>[2x]MTRTLPPGVSDERFDAALQRFRDVVGDKWVLSTADELEAFRDPYPVGAAEANLPSAVVSPESTEQVQDIVRIANEYGIPLSPVSTGKNNGYGGAAPRLSGSVIVKTGERMNRILEVNEKYGYALLEPGVTYFDLYEYLQSHDSGLMLDCPDLGWGSVVGNTLDRGVGYTPYGDHFMWQTGLEVVLPQGEVMRTGMGALPGSDAWQLFPYGFGPFPDGMFTQSNLGIVTKMGIALMQRPPASQSFLITFDKEEDLEQIVDIMLPLRINMAPLQNVPVLRNIFMDAAAVSKRTEWFDGDGPMPAEAIERMKKDLDLGFWNFYGTLYGPPPLIEMYYGMIKEAFGKIPGA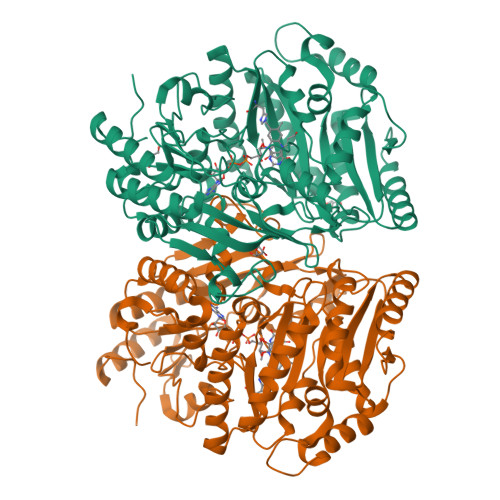RFFTHEERDDRGGHVLQDRHKINNGIPSLDELQLLDWVPNGGHIGFSPVSAPDGREAMKQFEMVRNRANEYNKDYAAQFIIGLREMHHVCLFIYDTAIPEAREEILQMTKVLVREAAEAGYGEYRTHNALMDDVMATFNWGDGALLKFHEKIKDALDPNGIIAPGKSGIWSQRFRGQNL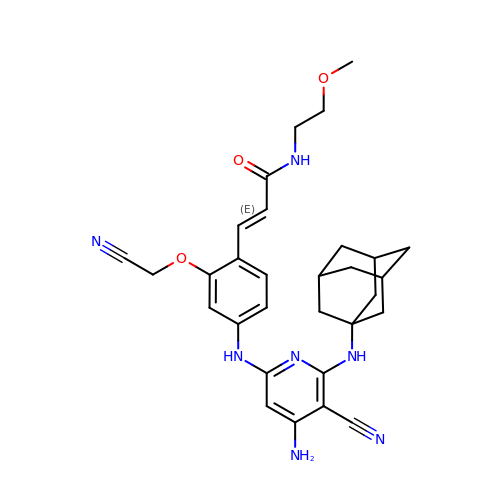(2E)-3-[4-({4-amino-5-cyano-6-[(3s,5s,7s)-tricyclo[3.3.1.1~3,7~]dec-1-ylamino]pyridin-2-yl}amino)-2-(cyanomethoxy)phenyl]-N-(2-methoxyethyl)prop-2-enamide | C30 H35 N7 O3 | XFGLTLTUEITKOH-SWLKYIRASA-N>AATYAQTLQNIPETNVTTLDNGLRVASEESSQPTCTVGVWIGAGSRYENEKNNGAGYFVEHLAFKGTKKRPCAAFEKEVESMGAHFNGYTSREQTAFYIKALSKDMPKVVELLADVVQNCALEESQIEKERGVILQELKEMDNDMTNVTFDYLHATAFQGTALARTVEGTTENIKHLTRADLASYIDTHFKAPRMVLAAAGGISHKELVDAARQHFSGVSFTYKEDAVPILPRCRFTGSEIRARDDALPVAHVALAVEGPGWADPDNVVLHVANAIIGRYDRTFGGGKHLSSRLAALAVEHKLCHSFQTFNTSYSDTGLFGFHFVADPLSIDDMMFCAQGEWMRLCTSTTESEVKRAKNHLRSAMVAQLDGTTPVCETIGSHLLNYGRRISLEEWDSRISAVDARMVRDVCSKYIYDKCPALAAVGPIEQLLDYNRIRSGMYWIRF[2x];>SLKVAPKVAVSAAAERVKLCPGAEDLEITKLPNGLIIASLENFSPASRIGVFIKAGSRYETTANLGTAHLLRLASPLTTKGASSFRITRGIEAVGGSLSVYSTREKMTYCVECLRDHVDTVMEYLLNVTTAPEFRPWEVTDLQPQLKVDKAVAFQSPQVGVLENLHAAAYKTALANPLYCPDYRIGKITSEQLHHFVQNNFTSARMALVGIGVKHSDLKQVAEQFLNI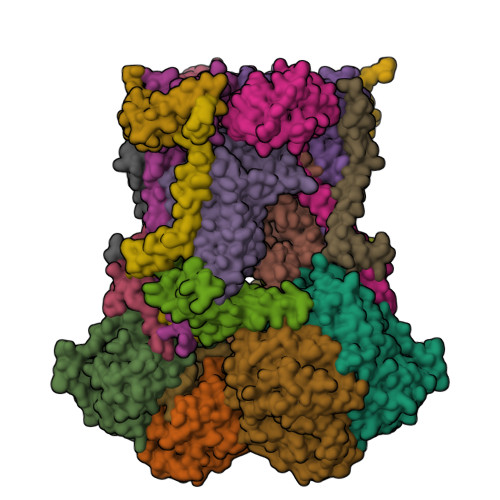RSGAGTSSAKATYWGGEIREQNGHSLVHAAVVTEGAAVGSAEANAFSVLQHVLGAGPLIKRGSSVTSKLYQGVAKATTQPFDASAFNVNYSDSGLFGFYTISQAAHAGEVIRAAMNQLKAAAQGGVTEEDVTKAKNQLKATYLMSVETAQGLLNEIGSEALLSGTHTAPSVVAQKIDSVTSADVVNAAKKFVSGKKSMAASGDLGSTPFLDEL[2x];>MAPNIRKSHPLLKMINNSLIDLPAPSNISAWWNFGSLLAVCLMTQILTGLLLAMHYTADTSLAFSSVAHTCRNVQYGWLIRNLHANGASFFFICIFLHIGRGLYYGSYLYKETWNTGVILLLTLMATAFVGYVLPWGQMSFWGATVITNLFSAIPYIGHTLVEWAWGGFSVDNPTLTRFFALHFLLPFAIAGITIIHLTFLHESGSNNPLGISSDSDKIPFHPYYSFKDILGLTLMLTPFLTLALFSPNLLGDPENFTPANPLVTPPHIKPEWYFLFAYAILRSIPNKLGGVLALAASVLILFLIPFLHKSKQRTMTFRPLSQTLFWLLVANLLILTWIGSQPVEHPFIIIGQMASLSYFTILLILFPTIGTLENKMLNY[2x];>GELELHPPAFPWSHGGPLSALDHSSVRRGFQVYKQVCSACHSMDYVAFRNLIGVTHTEAEAKALAEEVEVQDGPDENGELFMRPGKISDYFPKPYPNPEAARAANNGALPPDLSYIVNARHGGEDYVFSLLTGYCDPPAGVVVREGLHYNPYFPGQAIGMAPPIYNEILEYDDGTPATMSQIAKDVCTFLRWAAEPEHDQRKRMGLKMLLISALLTSLLYYMKRHKWSVLKSRKMAYRPPK[2x];>VHNDVTVPDFSAYRREDVMDATTSSQTSSEDRKGFSYLVTATACVATAYAAKNVVTQFISSLSASADVLALSKIEIKLSDIPEGKNVAFKWRGKPLFVRHRTQAEINQEAEVDVSKLRDPQHDLDRVKKPEWVILVGVCTHLGCVPIANSGDFGGYYCPCHGSHYDASGRIRKGPAPYNLEVPTYQFVGDDLVVVG[2x];>AARATVAGGGRLMDRIRKWYYNAAGFNKYGLMRDDTLYEDDDVKEALKRLPEDLYNERMFRIKRALDLSLKHRILPKEQWVKYEEDKPYLEPYLKEVIRERLEREAWNKK[2x];>[2x]GIHFGNLARVRHIITYSLSPFEQRAIPNIFSDALPNVWRRFSSQVFKVAPPFLGAYLLYSWGTQEFERLKRKNPADYENDQ;>[2x]LRGSGEEEEEELVDPLTTIREHCEQTEKCVKARERLELCDARVSSRSHTEEQCTEELFDFLHARDHCVAHKLFNKLK;>MLSVAARSGPFAPYLSAAAHAVPGPLXXXXXXXXXXXXXXXDLKRPLLCRESMSGRSARRDLVAGISLNAPASVRY[2x];>[2x]ALLRQAYSALFRRTSTFALTVVLGAVLFERAFDQGADAIFEHLNEGKLWKHIKHKYEASEE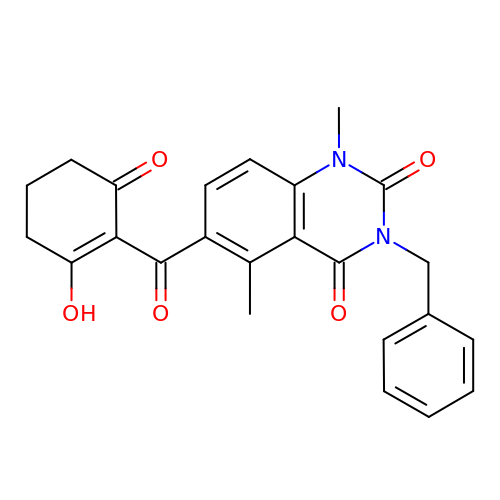1,5-dimethyl-6-(2-oxidanyl-6-oxidanylidene-cyclohexen-1-yl)carbonyl-3-(phenylmethyl)quinazoline-2,4-dione | C24 H22 N2 O5 | WOMKWUPMJGUMOM-UHFFFAOYSA-N> MRGSHHHHHHDDYDGIPNLTAVQISPNADPALGLEYPVRPPVPGAGGLNASAKGIHSIAIGATAEAAKGAAVAVGAGSIATGVNSVAIGPLS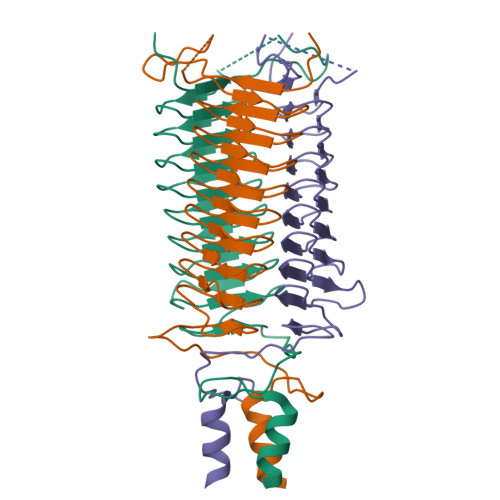KALGDSAVTYGAASTAQKDGVAIGARASTSDTGVAVGFNSKADAKNSVAIGHSSHVAANHGYSIAIGDRSKTDRENSVSIGHESLNRQLTHLAAGTKDTDAVNVAQLKKEIEKTQENTNKRSAELLANANAYAD> LPLDEHCERLPYDASKWEFPRDRLKLGKPLGRGAFGQVIEADAFGIDKTATCRTVAVKMLKEGATHSEHRALMSELKILIHIGHHLNVVNLLGACTKPGGPLMVIVEFCKFGNLSTYLRSKRNEFVPYKTKGARFRQGKDYVGAIPVDLKRRLDSITSSQSSASSGFVEEKSLSDVEEEEAPEDLYKDFLTLEHLICYSFQVAKGMEFLASRKCIHRDLAARNILLSEKNVVKICDFGLARD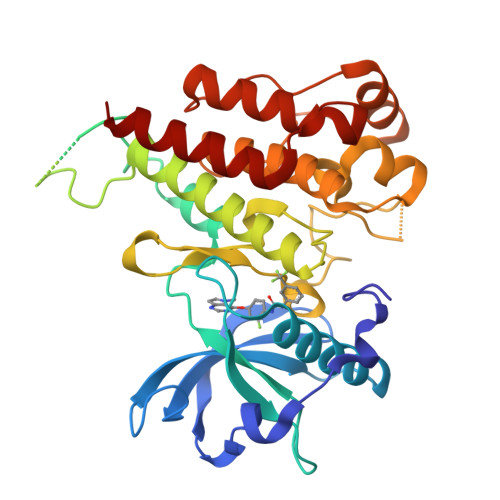IYKDPDYVRKGDARLPLKWMAPETIFDRVYTIQSDVWSFGVLLWEIFSLGASPYPGVKIDEEFCRRLKEGTRMRAPDYTTPEMYQTMLDCWHGEPSQRPTFSELVEHLGNLLQANAQ3-[(4-azanyl-6-methoxy-1,3,5-triazin-2-yl)amino]-4-[[(~{S})-[2,2-bis(fluoranyl)-1,3-benzodioxol-4-yl]-(3-chloranylpyridin-2-yl)methyl]amino]benzenesulfonamide 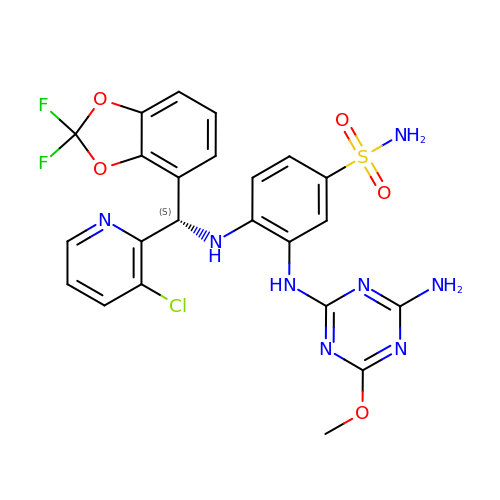| C23 H19 Cl F2 N8 O5 S | BAQOPDGRUNKWLM-KRWDZBQOSA-N> MEQAMRERSELARKGIARAKSVVALAYAGGVLFVAENPSRSLQKISELYDRVGFAAAGKFNEFDNLRRGGIQFADTRGYAYDRRDVTGRQLANVYAQTLGTIFTEQAKPYEVELCVAEVAHYGETKRPELYRITYDGSIADEPHFV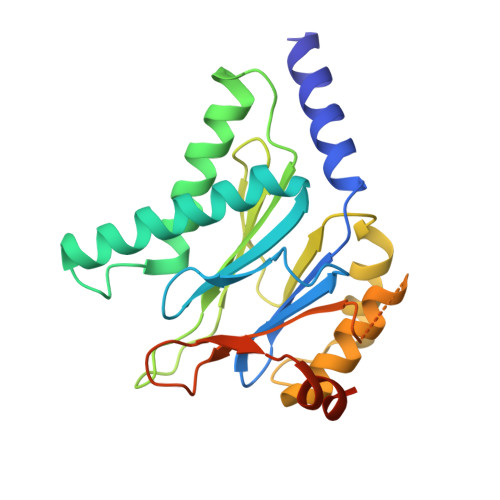VMGGTTEPIANALKESYAENASLTDALRIAVAALRAGSADTSGGDQPTLGVASLEVAVLDANRPRRAFRRITGSALQALLVDQESPQSDGESSG>[2x]MDYKDDDDKLAAANSSIDLISTSLYKKAGLTMVTGGGAAPPGTVTEPLPSVIVLSAGRKMAAAAAAASGPGCSSAAGAGAAGVSEWLVLRDGCMHCDADGLHSLSYHPALNAILAVTSRGTIKVIDGTSGATLQASALSAKPGGQVKCQYISAVDKVIFVDDYAVGCRKDLNGILLLDTALQTPVSKQDDVVQLELPVTEAQQLLSACLEKVDISSTEGYDLFITQLKDGLKNTSHETAANHKVAKWATVTFHLPHHVLKSIASAIVNELKKINQNVAALPVASSVMDRLSYLLPSARPELGVGPGRSVDRSLMYSEANRRETFTSWPHVGYRWAQPDPMAQAGFYHQPASSGDDRAMCFTCSVCLVCWEPTDEPWSEHERHSPNCPFVKGEHTQNVPLSVTLATSPAQFPCTDGTDRISCFGSGSCPHFLAAATKRGKICIWDVSKLMKVHLKFEINAYDPAIVQQLILSGDPSSGVDSRRPTLAWLEDSSSCSDIPKLEGDSDDLLEDSDSEEHSRSDSVTGHTSQKEAMEVSLDITALSILQQPEKLQWEIVANVLEDTVKDLEELGANPCLTNSKSEKTKEKHQEQHNIPFPCLLAGGLLTYKSPATSPISSNSHRSLDGLSRTQGESISEQGSTDNESCTNSELNSPLVRRTLPVLLLYSIKESDEKAGKIFSQMNNIMSKSLHDDGFTVPQIIEMELDSQEQLLLQDPPVTYIQQFADAAANLTSPDSEKWNSVFPKPGTLVQCLRLPKFAEEENLCIDSITPCADGIHLLVGLRTCPVESLSAINQVEALNNLNKLNSALCNRRKGELESNLAVVNGANISVIQHESPADVQTPLIIQPEQRNVSGGYLVLYKMNYATRIVTLEEEPIKIQHIKDPQDTITSLILLPPDILDNREDDCEEPIEDMQLTSKNGFEREKTSDISTLGHLVITTQGGYVKILDLSNFEILAKVEPPKKEGTEEQDTFVSVIYCSGTDRLCACTKGGELHFLQIGGTCDDIDEADILVDGSLSKGIEPSSEGSKPLSNPSSPGISGVDLLVDQPFTLEILTSLVELTRFETLTPRFSATVPPCWVEVQQEQQQRRHPQHLHQQHHGDAAQHTRTWKLQTDSNSWDEHVFELVLPKACMVGHVDFKFVLNSNITNIPQIQVTLLKNKAPGLGKVNALNIEVEQNGKPSLVDLNEEMQHMDVEESQCLRLCPFLEDHKEDILCGPVWLASGLDLSGHAGMLTLTSPKLVKGMAGGKYRSFLIHVKAVNERGTEEICNGGMRPVVRLPSLKHQSNKGYSLASLLAKVAAGKEKSSNVKNENTSGTRKSENLRGCDLLQEVSVTIRRFKKTSISKERVQRCAMLQFSEFHEKLVNTLCRKTDDGQITEHAQSLVLDTLCWLAGVHSNGPGSSKEGNENLLSKTRKFLSDIVRVCFFEAGRSIAHKCARFLALCISNGKCDPCQPAFGPVLLKALLDNMSFLPAATTGGSVYWYFVLLNYVKDEDLAGCSTACASLLTAVSRQLQDRLTPMEALLQTRYGLYSSPFDPVLFDLEMSGSSCKNVYNSSIGVQSDEIDLSDVLSGNGKVSSCTAAEGSFTSLTGLLEVEPLHFTCVSTSDGTRIERDDAMSSFGVTPAVGGLSSGTVGEASTALSSAAQVALQSLSHAMASAEQQLQVLQEKQQQLLKLQQQKAKLEAKLHQTTAAAAAAASAVGPVHNSVPSNPVAAPGFFIHPSDVIPPTPKTTPLFMTPPLTPPNEAVSVVINAELAQLFPGSVIDPPAVNLAAHNKNSNKSRMNPLGSGLALAISHASHFLQPPPHQSIIIERMHSGARRFVTLDFGRPILLTDVLIPTCGDLASLSIDIWTLGEEVDGRRLVVATDISTHSLILHDLIPPPVCRFMKITVIGRYGSTNARAKIPLGFYYGHTYILPWESELKLMHDPLKGEGESANQPEIDQHLAMMVALQEDIQCRYNLACHRLETLLQSIDLPPLNSANNAQYFLRKPDKAVEEDSRVFSAYQDCIQLQLQLNLAHNAVQRLKVALGASRKMLSETSNPEDLIQTSSTEQLRTIIRYLLDTLLSLLHASNGHSVPAVLQSTFHAQACEELFKHLCISGTPKIRLHTGLLLVQLCGGERWWGQFLSNVLQELYNSEQLLIFPQDRVFMLLSCIGQRSLSNSGVLESLLNLLDNLLSPLQPQLPMHRRTEGVLDIPMISWVVMLVSRLLDYVATVEDEAAAAKKPLNGNQWSFINNNLHTQSLNRSSKGSSSLDRLYSRKIRKQLVHHKQQLNLLKAKQKALVEQMEKEKIQSNKGSSYKLLVEQAKLKQATSKHFKDLIRLRRTAEWSRSNLDTEVTTAKESPEIEPLPFTLAHERCISVVQKLVLFLLSMDFTCHADLLLFVCKVLARIANATRPTIHLCEIVNEPQLERLLLLLVGTDFNRGDISWGGAWAQYSLTCMLQDILAGELLAPVAAEAMEEGTVGDDVGATAGDSDDSLQQSSVQLLETIDEPLTHDITGAPPLSSLEKDKEIDLELLQDLMEVDIDPLDIDLEKDPLAAKVFKPISSTWYDYWGADYGTYNYNPYIGGLGIPVAKPPANTEKNGSQTVSVSVSQALDARLEVGLEQQAELMLKMMSTLEADSILQALTNTSPTLSQSPTGTDDSLLGGLQAANQTSQLIIQLSSVPMLNVCFNKLFSMLQVHHVQLESLLQLWLTLSLNSSSTGNKENGADIFLYNANRIPVISLNQASITSFLTVLAWYPNTLLRTWCLVLHSLTLMTNMQLNSGSSSAIGTQESTAHLLVSDPNLIHVLVKFLSGTSPHGTNQHSPQVGPTATQAMQEFLTRLQVHLSSTCPQIFSEFLLKLIHILSTERGAFQTGQGPLDAQVKLLEFTLEQNFEVVSVSTISAVIESVTFLVHHYITCSDKVMSRSGSDSSVGARACFGGLFANLIRPGDAKAVCGEMTRDQLMFDLLKLVNILVQLPLSGNREYSARVSVTTNTTDSVSDEEKVSGGKDGNGSSTSVQGSPAYVADLVLANQQIMSQILSALGLCNSSAMAMIIGASGLHLTKHENFHGGLDAISVGDGLFTILTTLSKKASTVHMMLQPILTYMACGYMGRQGSLATCQLSEPLLWFILRVLDTSDALKAFHDMGGVQLICNNMVTSTRAIVNTARSMVSTIMKFLDSGPNKAVDSTLKTRILASEPDNAEGIHNFAPL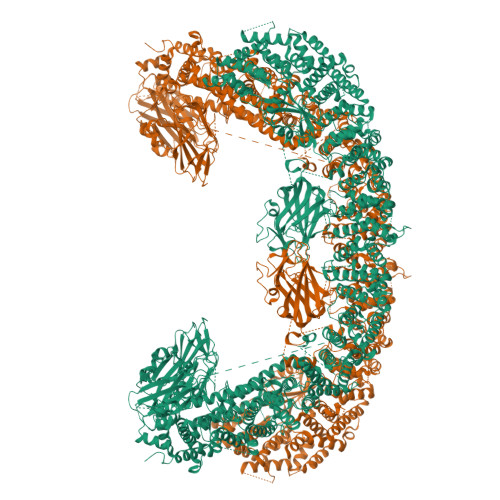GTITSSSPTAQPAEVLLQATPPHRRARSAAWSYIFLPEEAWCDLTIHLPAAVLLKEIHIQPHLASLATCPSSVSVEVSADGVNMLPLSTPVVTSGLTYIKIQLVKAEVASAVCLRLHRPRDASTLGLSQIKLLGLTAFGTTSSATVNNPFLPSEDQVSKTSIGWLRLLHHCLTHISDLEGMMASAAAPTANLLQTCAALLMSPYCGMHSPNIEVVLVKIGLQSTRIGLKLIDILLRNCAASGSDPTDLNSPLLFGRLNGLSSDSTIDILYQLGTTQDPGTKDRIQALLKWVSDSARVAAMKRSGRMNYMCPNSSTVEYGLLMPSPSHLHCVAAILWHSYELLVEYDLPALLDQELFELLFNWSMSLPCNMVLKKAVDSLLCSMCHVHPNYFSLLMGWMGITPPPVQCHHRLSMTDDSKKQDLSSSLTDDSKNAQAPLALTESHLATLASSSQSPEAIKQLLDSGLPSLLVRSLASFCFSHISSSESIAQSIDISQDKLRRHHVPQQCNKMPITADLVAPILRFLTEVGNSHIMKDWLGGSEVNPLWTALLFLLCHSGSTSGSHNLGAQQTSARSASLSSAATTGLTTQQRTAIENATVAFFLQCISCHPNNQKLMAQVLCELFQTSPQRGNLPTSGNISGFIRRLFLQLMLEDEKVTMFLQSPCPLYKGRINATSHVIQHPMYGAGHKFRTLHLPVSTTLSDVLDRVSDTPSITAKLISEQKDDKEKKNHEEKEKVKAENGFQDNYSVVVASGLKSQSKRAVSATPPRPPSRRGRTIPDKIGSTSGAEAANKIITVPVFHLFHKLLAGQPLPAEMTLAQLLTLLYDRKLPQGYRSIDLTVKLGSRVITDPSLSKTDSYKRLHPEKDHGDLLASCPEDEALTPGDECMDGILDESLLETCPIQSPLQVFAGMGGLALIAERLPMLYPEVIQQVSAPVVTSTTQEKPKDSDQFEWVTIEQSGELVYEAPETVAAEPPPIKSAVQTMSPIPAHSLAAFGLFLRLPGYAEVLLKERKHAQCLLRLVLGVTDDGEGSHILQSPSANVLPTLPFHVLRSLFSTTPLTTDDGVLLRRMALEIGALHLILVCLSALSHHSPRVPNSSVNQTEPQVSSSHNPTSTEEQQLYWAKGTGFGTGSTASGWDVEQALTKQRLEEEHVTCLLQVLASYINPVSSAVNGEAQSSHETRGQNSNALPSVLLELLSQSCLIPAMSSYLRNDSVLDMARHVPLYRALLELLRAIASCAAMVPLLLPLSTENGEEEEEQSECQTSVGTLLAKMKTCVDTYTNRLRSKRENVKTGVKPDASDQEPEGLTLLVPDIQKTAEIVYAATTSLRQANQEKKLGEYSKKAAMKPKPLSVLKSLEEKYVAVMKKLQFDTFEMVSEDEDGKLGFKVNYHYMSQVKNANDANSAARARRLAQEAVTLSTSLPLSSSSSVFVRCDEERLDIMKVLITGPADTPYANGCFEFDVYFPQDYPSSPPLVNLETTGGHSVRFNPNLYNDGKVCLSILNTWHGRPEEKWNPQTSSFLQVLVSVQSLILVAEPYFNEPGYERSRGTPSGTQSSREYDGNIRQATVKWAMLEQIRNPSPCFKEVIHKHFYLKRVEIMAQCEEWIADIQQYSSDKRVGRTMSHHAAALKRHTAQLREELLKLPCPEGLDPDTDDAPEVCRATTGAEETLMHDQVKPSSSKELPSDFQL golvatinib  | 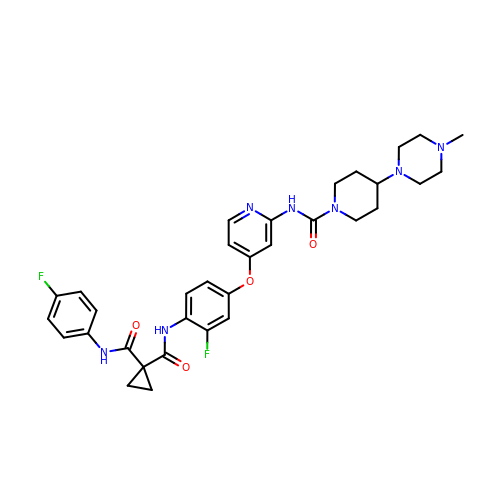C33 H37 F2 N7 O4 | UQRCJCNVNUFYDX-UHFFFAOYSA-N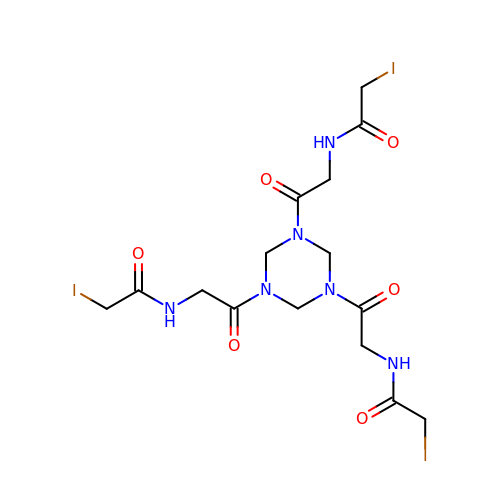N-[2-[3,5-bis[2-(2-iodanylethanoylamino)ethanoyl]-1,3,5-triazinan-1-yl]-2-oxidanylidene-ethyl]-2-iodanyl-ethanamide | C15 H21 I3 N6 O6 | NQXMSMNRHYWXDM-UHFFFAOYSA-N>MSHVEYSRITKFFQEQPLEGYTLFSHRSAPNGFKVAIVLSELGFHYNTIFLDFNLGEHRAPEFVSVNPNARVPALIDHGMDNLSIWESGAILLHLVNKYYKETGNPLLWSDDLADQSQINAWLFFQTSGHAPMIGQALHFRYFHSQKIASAVERYTDEVRRVYGVVEMALAERREALVMEL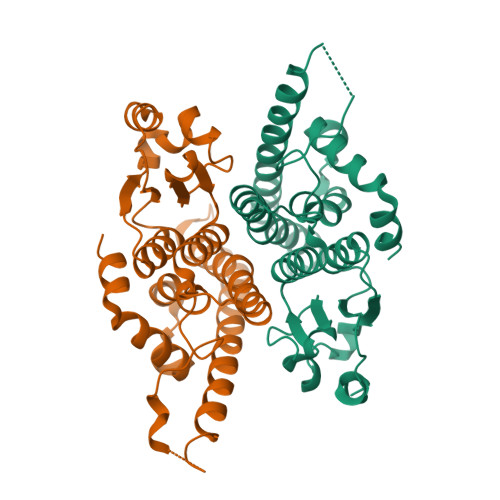DTENAAAYSAGTTPMSQSRFFDYPVWLVGDKLTIADLAFVPWNNVVDRIGINIKIEFPEVYKWTKHMMRRPAVIKALRGE[4x]>MTAVSEFRPGLEGVPATLSSISFVDGQRGVLEYRGISIEQLAQQSSFLETAYLLIWGHLPTQQELTEFEHEIRYHRRIKFRIRDMMKCFPDSGHPMDALQASAAALGLFYSRRALDDPEYIRAAVVRLLAKIPTMVAAFQLIRKGNDPIQPRDELDYAANFLYMLTEREPDPVAARIFDICLTLHAEHTINASTFSAMVTASTLTDPYAVVASAVGTLAGPLHGGANEEVLDMLEAIGSVENVEPYLDHCIATKTRIMGFGHRVYKVKDPRAVILQNLAEQ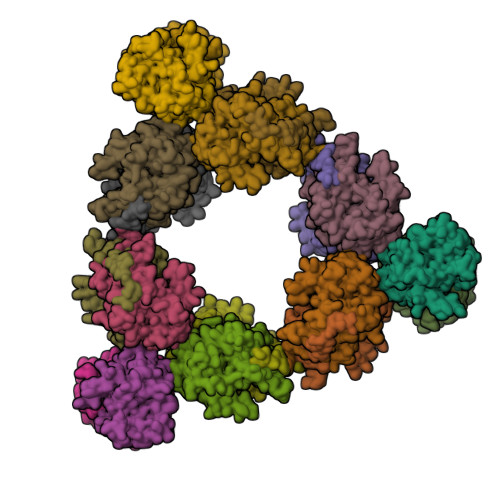LFDIFGHDPYYEIAVAVEKAAAERLSHKGIYPNVDFYSGLVYRKLGIPSDLFTPVFAIARVAGWLAHWKEQLNENRIFRPTQIYTGSRNLDYTPIADRDLAIESDLEHHHHHH[18x]> MANVNKVVRRRQVALLIALVLGIGAGGAGTWMVSEMNLKKAPPAKAPKGEPAPDMTGVVNQSFDNKVQRSAIAEAQRLNKETQTEIKKLRTEMGLVSRDLKGSQDRIRELEDQNQLLQTQLEAGKNFDSLSAEPLPGALASQGKPAPAGNVPPPTSFWPA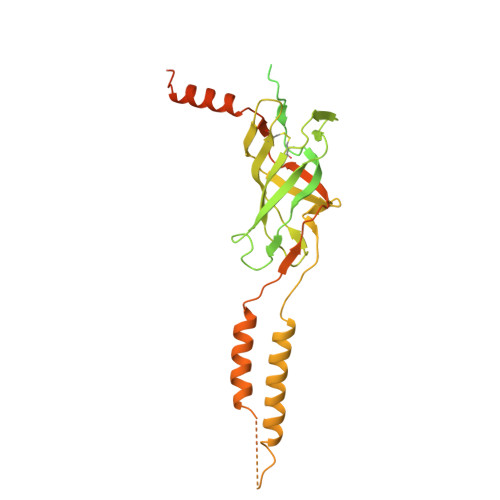GGGQAPAAPVMTPIQRPGMMDSQEFSLPDTGPKKPRFPWISSGSFVEAIVVEGADANASVTGDKNTAPMQLRLTGKVQMPNDEEFDLTGCFVTLEAWGDVSSERAIVRSRSISCKLGDDDIDQKIAGHVSFMGKNGIKGEVVMRNGQILLYAGGAGFLDGIGKGIEKASSTTVGVGATASMSAADIGQAGLGGGVSSAAKTLSDYYIKRAEQYHPVIPIGAGNEVTLVFQDGFQLETLEEARAKAAARKKQNQPSASSTPAAMPGNTPDMLKQLQDFRVGDTVDPATGQVVTQ> MGSLHMIDYKEIEVEEVVGRGAFGVVCKAKWRAKDVAIKQIESESERKAFIVELRQLSRVNHPNIVKLYGACLNPVCLVMEYAEGGSLYNVLHGAEPLPYYTAAHAMSWCLQCSQGVAYLHSMQPKALIHRDLKPPNLLLVAGGTVLKICDFGTACDIQTHMTNNKGSAAWMAPE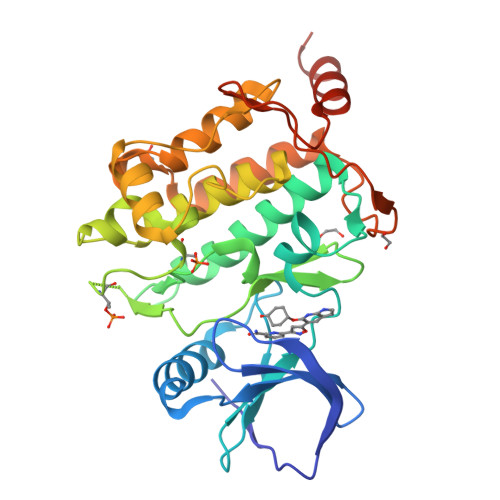VFEGSNYSEKCDVFSWGIILWEVITRRKPFDEIGGPAFRIMWAVHNGTRPPLIKNLPKPIESLMTRCWSKDPSQRPSMEEIVKIMTHLMRYFPGADEPLQYPCQHSLPPGEDGRVEPYVDFAEFYRLWSVDHGEQSVVTAP> PGSAPDFSRNPMKKMVQVQVGSLVILDCKPRASPRALSFWKKGDMMVREQARVSFLNDGGLKIMNVTKADAGTYTCTAENQFGKANGTTHLVVTEPTRIILAPSNMDVAVGESVILPCQVQHDPLLDIMFAWYFNGALTDFKKDGSHFEKVGGSSSGDLMIRNIQLKHSGKYVCMVQTGVDSVSSAAELIVRGSPGPPENVKVDEITDTTAQLSWTEGTDSHSPVISYAVQARTPFSVGWQSVRTVPEVIDGKTHTATVVELNPWVEYEFRIVASNKIGGGEPSLPSEKVRTEEAAPEIAPSEVSGGGGSRSELVITWDPVPEELQNGGG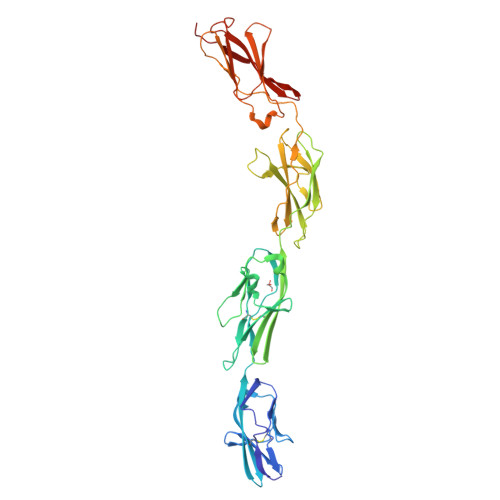FGYVVAFRPLGVTTWIQTVVTSPDNPRYVFRNESIVPFSPYEVKVGVYNNKGEGPFSPVTTVFSAEEE3-aminopropan-1-ol | C3 H9 N O | 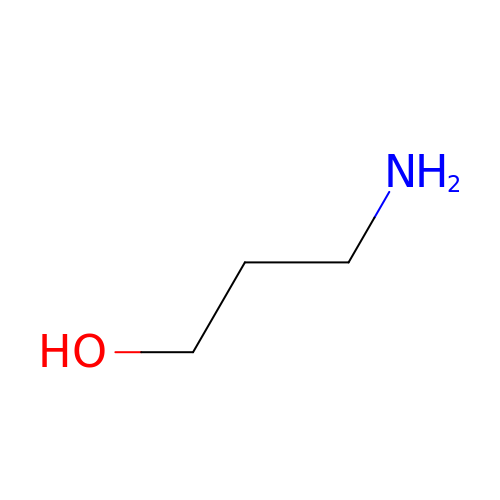WUGQZFFCHPXWKQ-UHFFFAOYSA-N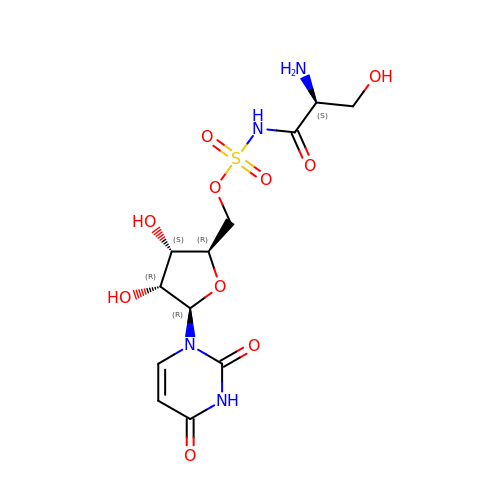5'-O-(N-(L-seryl)-Sulfamoyl)uridine | C12 H18 N4 O10 S | QIOFKSOPWDKKDG-DANLAGSESA-N>ETLVRPKPLLLKLLKSVGAQKDTYTMKEVLFYLGQYIMTKRLYDEKQQHIVYCSNDLLGDLFGVPSFSVKEHRKIYTMIYRNLVV[2x];>DWWPLAFEALL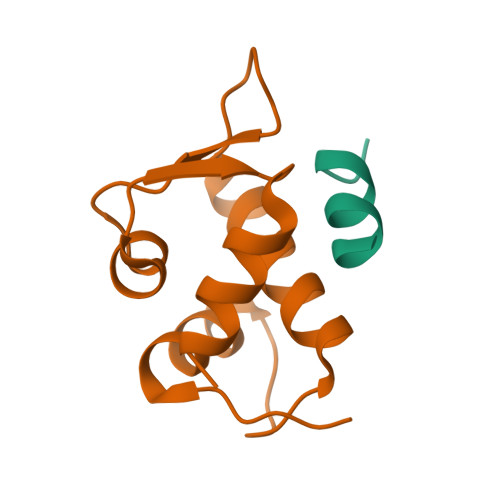R[2x]>MVQEIDLGLTCDMHVHVREGAMCELVTPKIRDGGVSIAYIMPNLQPPITTLDRVIEYKKTLQKLAPKTTFLMSFYLSKDLTPDLIHEAAQQHAIRGVKCYPAGVTTNSAAGVDPNDFSAFYPIFKAMQEENLVLNLHGEKPSVHDGDKEPIHVLNAEEAFLPALKKLHNDFPNLKIILEHCTSESAIKTIEDINKNVKKATDVKVAATLTAHHLFLTIDDWAGNPVNFCKPVAKLPNDKKALVKAAVSGKPYFFFGSDSAPHPVQNKANYEGVCAGVYSQSFAIPYIAQVFEEQNALENLKGFVSDFGISFYEVKDSEVASSDKAILFKKEQVIPQVISDGKDISIIPFKAGDKLSWSVRWEPRLEHHHHHH[4x]

Dihydroorotase (DHOase) is a zinc metalloenzyme that catalyzes the reversible cyclization of N-carbamoyl aspartate (CA-asp) to dihydroorotate (DHO) in the third step of the pathway for the biosynthesis of pyrimidine nucleotides. Dihydroorotase (DHOase) possesses a binuclear metal center in which two Zn ions are bridged by a posttranslationally carbamylated lysine. Crystal structures of ligand-bound DHOase show that the flexible loop extends toward the active site when CA-asp is bound (loop-in mode) or moves away from the active site, facilitating the product DHO release (loop-out mode). In bacteria and yeast, DHOase is monofunctional and belongs to the type II enzyme.

Thus, we incubated 5-FOA with the crystal of the ScDHOase-malate complex and obtained the crystal of the ScDHOase-5-FOA complex successfully. The crystal structure of ScDHOase complexed with 5-FOA was solved at 2.5 Å resolution. An asymmetric unit of the crystal contained four crystallography-independent ScDHOase monomers. The global architecture of each ScDHOase monomer showed a TIM-barrel structure and consisted of 15 α-helices, 12 β-sheets, 2 Zn ions, and 1 5-FOA molecule. The dimetal center (Znα/Znβ) in ScDHOase containing 4 His (i.e., H14, H16, H137, and H180), 1 Asp (i.e., D258), and 1 carbamylated Lys (i.e., Kcx98) was still self-assembled. The structure revealed a long flexible loop in each subunit which extended toward the active site when 5-FOA was bound. For ScDHOase, the carboxylate group of 5-FOA ligated the Zn atoms rather than interacting with the positively charged side chain of Arg18 as that in EcDHOase and huDHOase. The bound 5-FOA by ScDHOase adopted the reverse orientation compared with those by EcDHOase and huDHOase. According to our structure, Arg18, Asn43, His262, Thr105, Thr106, and Lys230 of ScDHOase were involved in the 5-FOA binding. Despite having a similar active site, the 5-FOA binding pose and the conformation of the catalytic loop of ScDHOase for 5-FOA binding (via the loop-in mode) differed from those of EcDHOase and huDHOase (via the loop-out mode).>IDMYLYDDNEESQVQFVGFVGEHSRYDLMLVHTNRHYGKTLVLNMQTNKFGIIGTDDLKEEGYIAHILGVNAEEGDEITEYLNEVIHL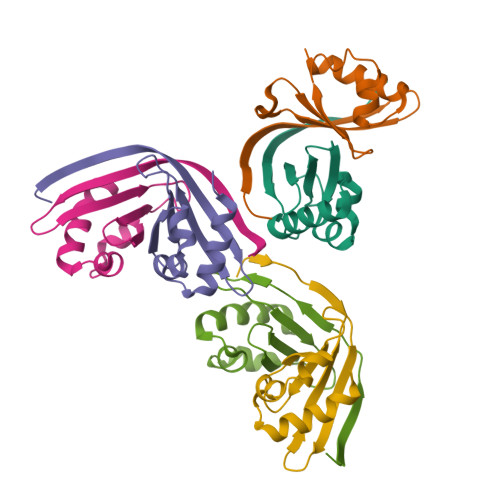E[6x]>MGCQSTQLQTPAPDTGGIVELNRQLGRGVNLGNALEAPWEGAWGVRLEEGFFELIREAGFKTIRLPVSWTHHAGRAAPYTIDPAFFSRVDWAVTQATRRGLNIVVNVHHYDELNANPQAEEARYLSIWRQIAERYRNQPGSVYFELLNEPHGRFNDNPQLWNDLLAKALRVVRESNPSRAVIVGPVGWNSLWRLSELRLPDDPNLIVTFHYYDPLEFTHQGAEWLNPVPPTGVVWRENQGAFAAGWQNWSWGSRVGFVGEALEITYQEGWAGFYLHSDAGVEGYDRLAFRTSAPVSLQ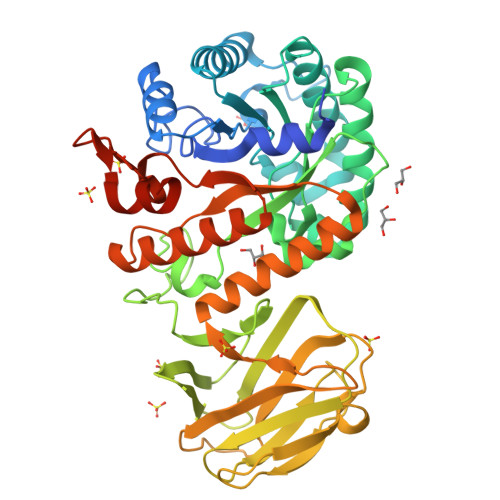VSCRRDAPAKAVTTSGGVETVVNLSECGNPSRLTDLILQNNSPNARAAFRLERLELRGPGSPLALLTHQQNAIAQAMEFAQRWAEQNRRPIFVGQFGAYEKGDLDSRVRWTGAVRSELEKRNFSWAYWEFAAGFGIYDRTTRQWRTPLLKALVPEQPKLAAALEHHHHHH[2x]>NIDTMAKALTTMQEQIDSLAAVVLQNRRGLDMLTAAQGGICLA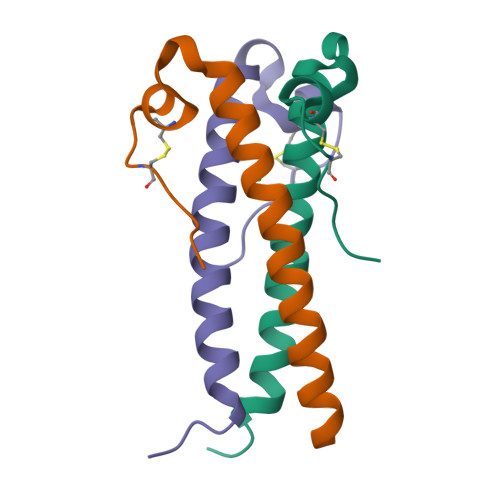LDEKCCFWVN[3x]> IVGGYTCQENSVPYQVSLNSGYHFCGGSLINDQWVVSAAHCYKSRIQVRLGEHNINVLEGNEQFVNAAKIIKHPNFDRETYNNDIMLIKLSSPVKLNARVATVALPSSCAPAGTQCLISGWGNTLSSGVNEPDLLQCLDAPLLPQADCEASYPGKITDNMVCVGFLEGGKDSCQGDSGGPVVCNGELQGIVSWGYGCALPDNPGVYTK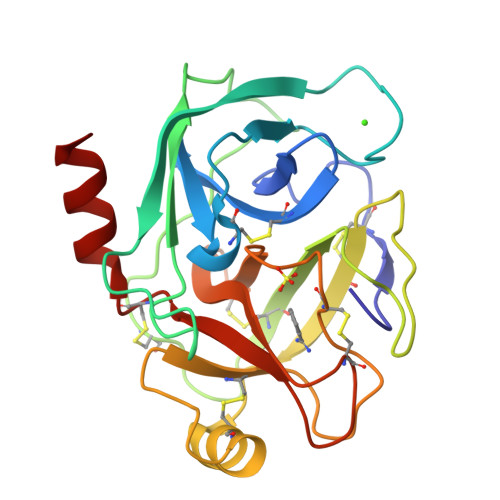VCNYVDWIQDTIAAN>MHHHHHHLPNITILATGGTIAGGGDSATKSNYTVGKVGVENLVNAVPQLKDIANVKGEQVVNIGSQDMNDNVWLTLAKKINTDCDKTDGFVITHGVDTMEETAYFLDLTVKCDKPVVMVGAMRPSTSMSADGPFNLYNAVVTAADKASANRGVLVVMNDTVLDGRDVTTTNTTDVATFKSVNYGPLGYIHNGKIDYQRTPARKHTSDTPFDVSKLNELPKVGIVYNYANASDLPAKALVDAGYDGIVSAG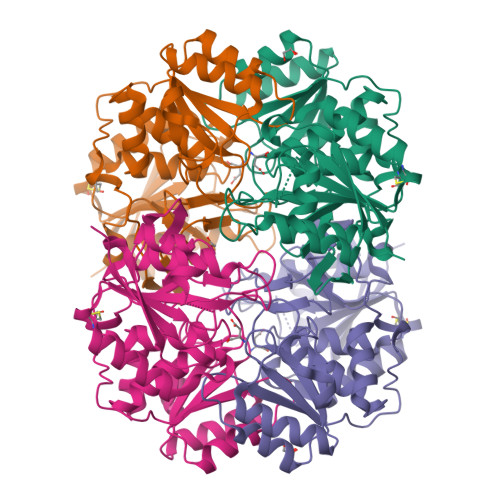VGNGNLYKSVFDTLATAAKTGTAVVRSSRVPTGATTQDAEVDDAKYGFVASGTLNPQKARVLLQLALTQTKDPQQIQQIFNQY[4x]> KAVTFYEDINYGGASVSLQPGNYTLSQLNTAKIPNDWMTSLKVPSGWTVDV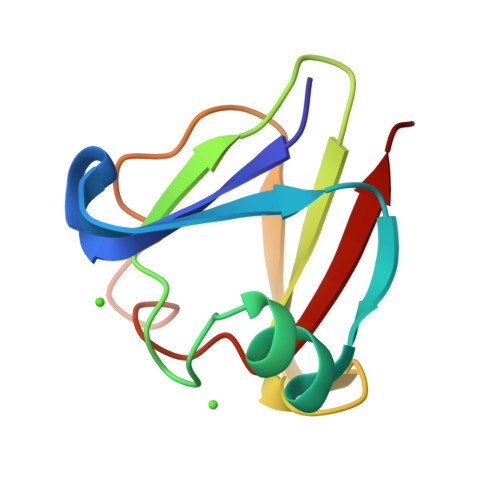YENDNFTGTKWTYTSDTPWVGNDANDKMTSVKIYST1-pentyl-4-phenyl-imidazol-2-amine | C14 H19 N3 | 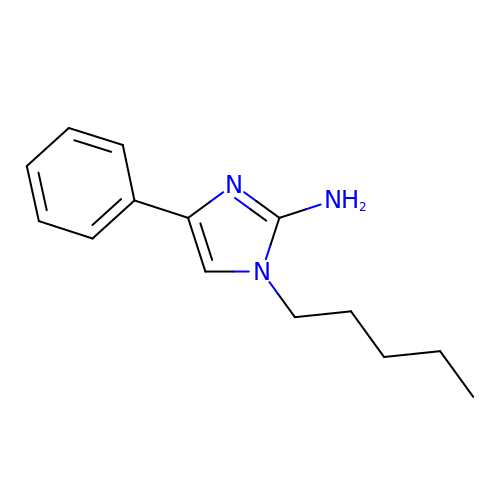NTJHSIKKNQRLPN-UHFFFAOYSA-N>[2x]MPEEMDKPLISLHLVDSDSSLAKVPDEAPKVGILGSGDFARSLATRLV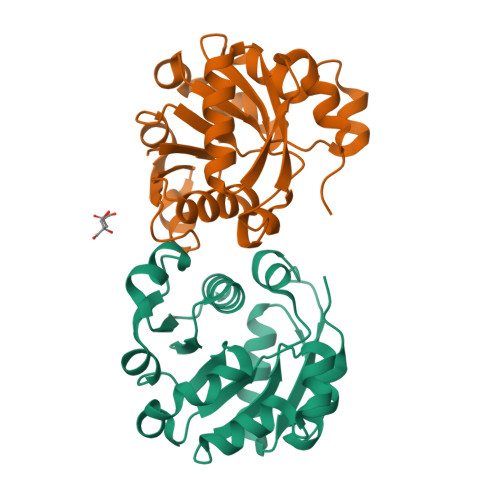GSGFKVVVGSRNPKRTARLFPSAAQVTFQEEAVSSPEVIFVAVFREHYSSLCSLSDQLAGKILVDVSNPTEQEHLQHRESNAEYLASLFPTCTVVKAFNVISAWTLQAGPRDGNRQVPICGDQPEAKRAVSEMALAMGFMPVDMGSLASAWEVEAMPLRLLPAWKVP>[2x]TFRRLWPTIAPFKAGLIVAGVALILNAASDTFMLSLLKPLLD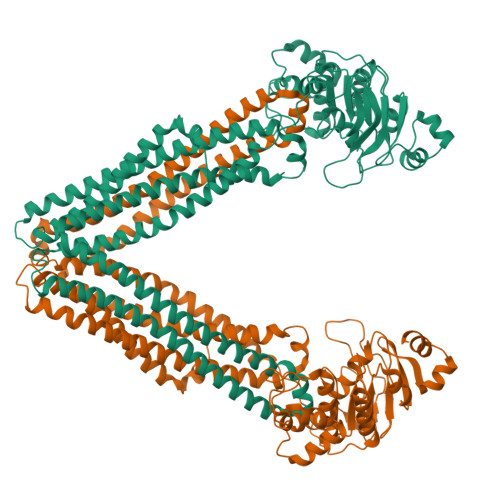DGFGKTDRSVLVWMPLVVIGLMILRGITSYVSSYCISWVSGKVVMTMRRRLFGHMMGMPVSFFDKQSTGTLLSRITYDSEQVASSSSGALITVVREGASIIGLFIMMFYYSWQLSIILIVLAPIVSIAIRVVSKRFRNISKNMQNTMGQVTTSAEQMLKGHKEVLIFGGQEVETKRFDKVSNRMRLQGMKMVSASSISDPIIQLIASLALAFVLYAASFPSVMDSLTAGTITVVFSSMIALMRPLKSLTNVNAQFQRGMAACQTLFTILDSEQEKDEGKRVIERATGDVEFRNVTFTYPGRDVPALRNINLKIPAGKTVALVGRSGSGKSTIASLITRFYDIDEGEILMDGHDLREYTLASLRNQVALVSQNVHLFNDTVANNIAYARTEQYSREQIEEAARMAYAMDFINKMDNGLDTVIGENGVLLSGGQRQRIAIARALLRDSPILILDEATSALDTESERAIQAALDELQKNRTSLVIAHRLSTIEKADEIVVVEDGVIVERGTHNDLLEHRGVYAQLHKMQF>[3x]TRDFNGTWEMESNENFEGYMKALDIDFATRKIAVRLTFTDVIDQDGDNFKTKATSTHLNYDVDFTVGVEFDEYTKSLDNRHVKALVTWEGDVLVCVQKGEKEN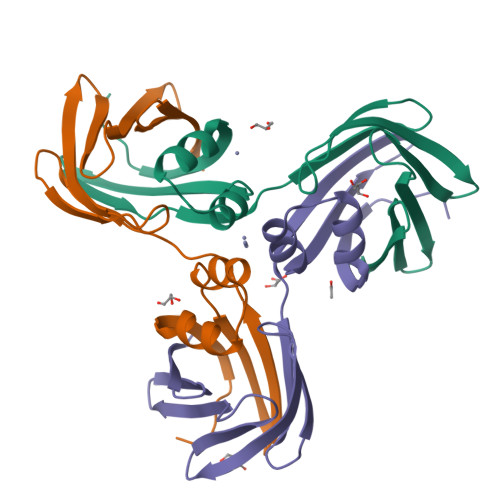RGWKKWIEGDKLYLELTCGDQVCRQVFKKK(7R)-8-cyclopentyl-7-(cyclopentylmethyl)-2-[(3,5-dichloro-4-hydroxyphenyl)amino]-5-methyl-7,8-dihydropteridin-6(5H)-one 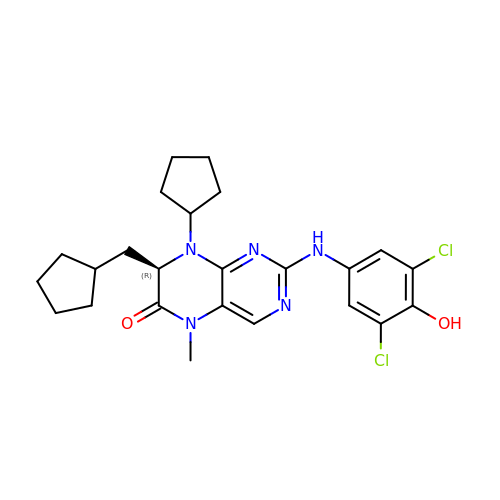| C24 H29 Cl2 N5 O2 | AEZJZTFWCDAUDF-LJQANCHMSA-N>[2x]MEDGAQMRVVAFGDQTYDCSEAVSQLLRVRDDAIVVDFLERAPAVLKAELARLSSEQQEETPRFATLAELVPRYRAGTLNPAVSQALTCIAQLGLFIRQHSSGQEAYPTAHDSCITGVCTGALTAVAVGSASSVTALVPLALHTVAVAVRLGARAWEIGSCLADARRGANGRYASWTSAVGGISPQDLQDRISAYTAEQALASVSVPYLSAAVGPGQSSVSAAPVILDAFLSTLLRPLTTTRLPITAPYHAPHLFTAKDVQHVTDCLPPSEAWPTVRIPIISFSRDEAVSRGASFPAAMSEAVRDCLIRPIALDRMAVSIANHARDLGKDSVLPSPIALSFSDKLGPQVNSHLPGAKAPTPELTSKSIPSAIGAEQQPMAKSPIAILAASGRFPQSSSMDQFWDVLINGVDTHELVPPTRWNAATHVSEDPKAKNVSGTGFGCWLHEAGEFDAAYFNMSPREAPQVDPAQRLALLTATEALEQAGVVPNRTSSTQKNRVGVWYGATSNDWMETNSAQNVDTYFIPGGNRAFIPGRVNYFHKFSGPSYTIDTACSSSLAALHMACNALWRGEVDTAIVGGTNVLTNPDMTAGLDAGHFLSRSGNCKTFDDEADGYCRGEAVVTLILKRLPDAQADKDPIQASILGIATNHSAEAASITRPHAGAQQDLFQQVLTETGLTANDISVCEMHGTGTQAGDSGETTSVVETLAPLNRSGSAVRTTPLYIGAVKSNVG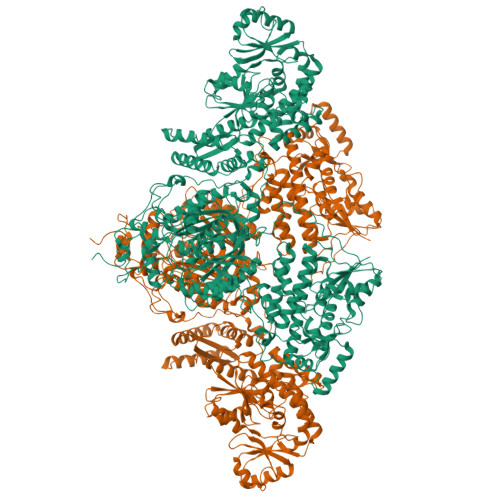HAESAAGVSSLAKILLMLKHSKIPPHVGIKTKLNHRLPDLAARNTHIARSEVPWPRPKNGKRRVLLNNFSAAGGNTCLVLEDAPEPEDSQEVDPREHHIVALSAKTPDSMVNNLTNMITWIDKHSGDSLATLPQLSYTTTARRVHHRHRAVATGTDLLQIRSSLQEQLDRRVSGERSIPHPPNGPSFVLAFTGQGSAFAGMGVDLYKRFASFRSDIARYDQICEGMSLPSIKAMFEDEKVFSTASPTLQQLTHVCFQMALYRLWKSLGVQAKAVVGHSLGEYAALYAAGVLSQSDTLYLVGRRAQLMEKHLSQGTHAMLAVRAKEEAIVAAIDGPPGEAYEFSCRNGEQRNVLGGTVAQIQAAKAALEAKKIRCQYLDTPMAFHTGQVDPILPELLQVAAACSIQDPQIPVISPAYGKVIRSAKDFQPEYFTHHCRSSVNMVDALQSAVEEGLLDKNVIGLEIGPGPVVTQFVKEAVGTTMQTFASINKDKDTWQLMTQALAKFYLAGASVEWSRYHEDFPGAQKVLELPAYGWALKNYWLQYVNDWSLRKGDPAVVVAASAAALEHHHHHH>[4x]MHADEVWPGLYLGDQDMANNRRELRRLGITHVLNASHSRWRGTPEAYEGLGIRYLGVEAHDSPAFDMSIHFQTAADFIHRALSQPGGKILVHSAVGVSRSATL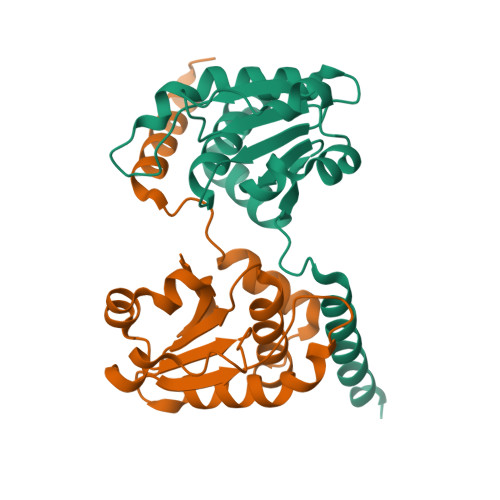VLAYLMLYHHLTLVEAIKKVKDHRGIIPNRGFLRQLLALDRRLRQGLEALEHHHHHH> NCDIH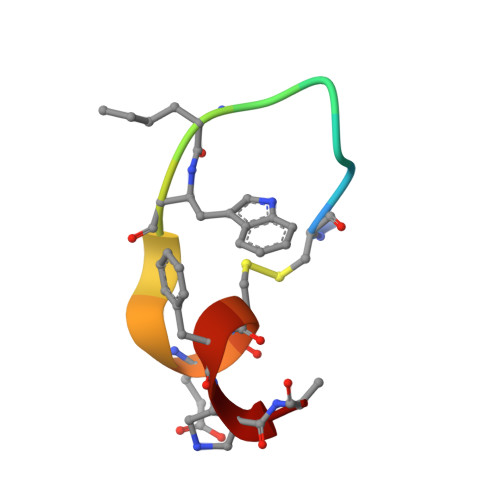VLWEWECFXR> TDKRKDGSGKLLYCSFCGKSQHEV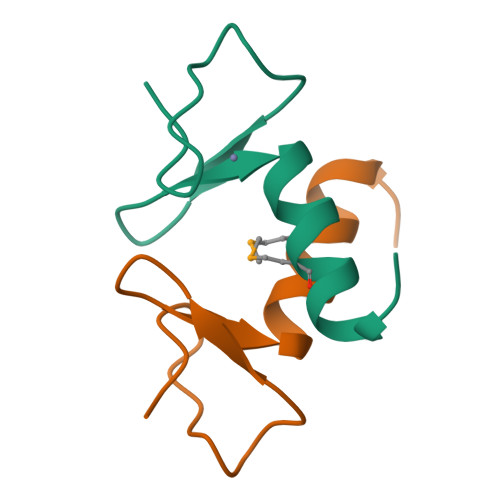RKLIAGPSVYICDECVDLMNDIIREEI> GAMAPIITQSVEVDLPDATESQAVSSNDNPPVIVEVSGIGQYTVVVEKD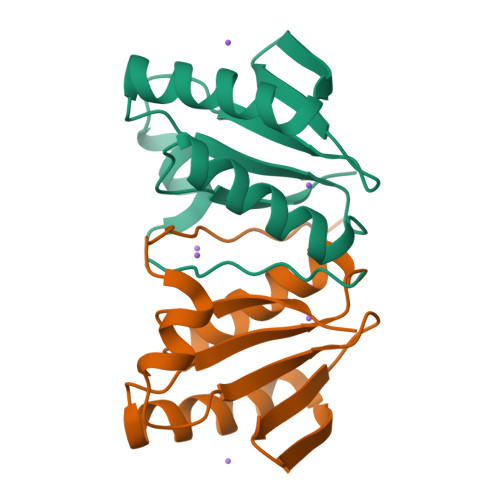RLERLPPEQVVAEVSSRFKANPKTVFLIGGAKDVPYDEIIKALNLLHSAGVKSVGLMTQPI> SQINQVRPKLPLLKILHAAGAQGEMFTVKEVMHYLGQYIMVKQLYDQQEQHMVYCGGDLLGELLGRQSFSVKDPS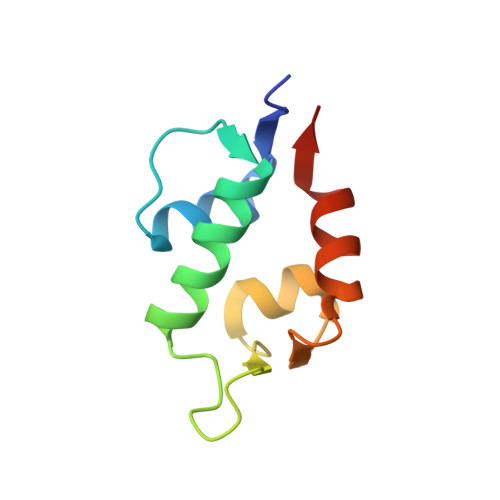PLYDMLRKNLVTLAT>[2x]MSLASNKKYTFACLLPKHLEGEYWTDVQKGIREAVTTYSDFNISANITHYDPYDYNSFVATSQAVIEEQPDG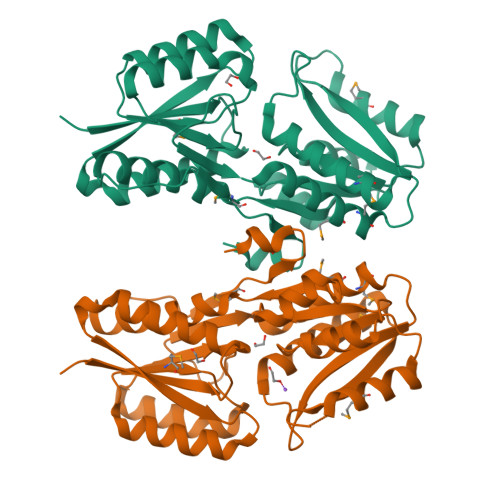VMFAPTVPQYTKGFTDALNELGIPYIYIDSQIKDAPPLAFFGQNSHQSGYFAARMLMLLAVNDREIVIFRKIHEGVIGSNQQESREIGFRQYMQEHHPACNILELNLHADLNIEDSRMLDDFFREHPDVKHGITFNSKVYIIGEYLQQRRKSDFSLIGYDLLERNVTCLKEGTVSFLIAQQPELQGFNSIKTLCDHLIFRKEVACTNYMPIDLLTKENIDYYHSEGHHHHHH>GGUCACAACGGCUUCCUGGCGUGACC[6x];>AUU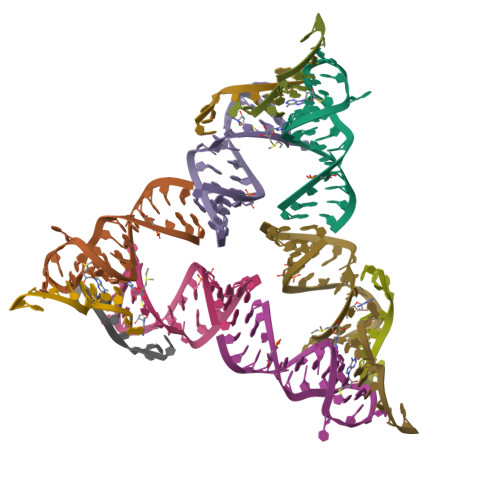GGAGCA[6x]> MVTFMITSALHRAADWAKSVFSSAALGDPRRTARLVNVAAQLAKYSGKSITISSEGSKAAQEGAYRFIRNPNVSAEAIRKAGAMQTVKLAQEFPELLAIEDTTSLSYRHQVAEELGKLGSIQDKSRGWWVHSVLLLEATTFRTVGLLHQEWWMRPDDPADADEKESGKWLAAAATSRLRMGSMMSNVIAVCDREADIHAYLQDKLAHNERFVVRSKHPRKDVESGLYLYDHLKNQPELGGYQISIPQKGVVDKRGKRKNRPARKASLSLRSGRITLKQGNITLNAVLAEEINPPKGETPLKWLLLTSEPVESLAQALRVIDIYTHRWRIEEFHKAWKTGAGAERQRMEEPDNLERMVSILSFVAVRLLQLRESFTPPQALRAQGLLKEAEHVESQSAETVLTPDECQLLGYLDKGKRKRKEKAGSLQWAYMAIARLGGFMDSKRTGIA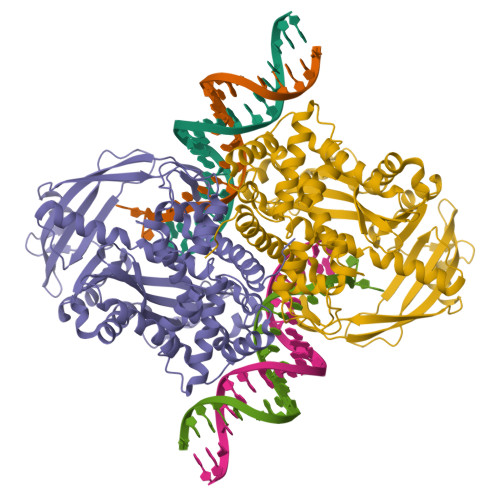SWGALWEGWEALQSKLDGFLAAKDLMAQGIKIG> GSTLTYPFHDWSQELSPRYAQLRASDAPVCPVVSEGTGDPLWLVTRYATAVKLLEDSRFSSEAAIASGAPRQEPVELRAPGTRGDGIAMLREAGLRSVLADGLGPRAVRRHQGWINDLAETLMSELASREGTFDLAADFVEPLSSALVSRTLLGELSADERDLLAHCADTGLRFCGVTHEEQVHAFTQMHEFFLEHARRLAGTPGEHLLKLIAEAPVDQGPLSDEALAEAGSLLVVAGFPTSSGFLCGALLTLLRHPDAVQELHAHPERVPSAVEELLRYTPLSTGSVKRMATE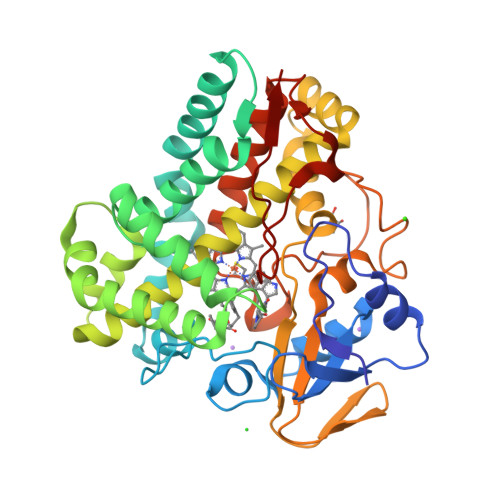DLEIDGVRIKAGEVVMVSLEAVNHDPDAFEDPDVFRPGREGPMHFGFGRGRHFCPGNRLARCVIEATVRAVARRPGLRLAVAPEEISWHEGLFFRRPRAIPATW>SNAMTVKPELNEITPYLQFNRQQWGNFRKDTPLTLTESDLDKLQGQIEIVSLKEVTEIYLPLSRLLSFYVTARQTLQQATYQFLGKPEPKVPYIIGIAGSVAVGKSTTSRVLKALLSRWPDHPNVEVITTDGFLYSNAKLEKQGLMKRKGFPESYDMPSLLRVLNAIKSGQRNVRIPVYSHHYYDIVRGQYEIVDQPDIVILEGLNILQTGVRKTLQQLQVFVSDFF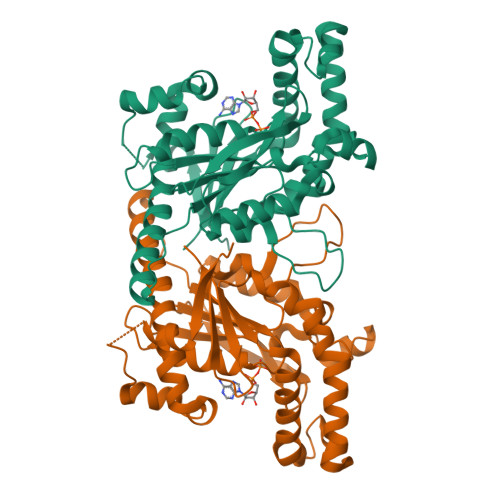DFSLFVDAQAQVIQKWYIDRVLSFWRTTFKDPHSYFHYLTQMSETEVAAFAKHVWNEINKVNLMENILPYKNRAQLILEKAADHSIQKVYLRKI[2x]>[2x]VSEPTTVAFDVRPGGVVHSFSHNVGPGDKYTCMFTYASQGGTNEQWQMSLGTSEDHQHFTCTIWRPQGKSYLYFTQFKAEVRGAEIEYAMAYSKAAFERESDVPLKTEEFEVTKTAVAHRPGAFKAELSKLVIVAKASRTEL

MYDGF, previously named c19orf10 (chromosome 19 open reading frame 10), is a poorly characterized protein, which was identified as a paracrine-acting protein that is secreted by monocytes and macrophages. Human MYDGF has 142 amino acids and consists of an N-terminal 31-residue-long signal peptide and the MYDGF protein sequence containing a C-terminal KDEL-like ER retention sequence. According to its primary amino acid sequence, MYDGF does not belong to any known cytokine or growth factor family. Treatment with recombinant MYDGF helps to protect and repair the heart after acute MI.

Recombinant full-length MYDGF, lacking the N-terminal signal peptide, was crystallized using sitting-drop vapor diffusion methods. MYDGF crystals diffracted to 1.6 Å. Due to the lack of initial start models, the structure of MYDGF was determined by Hg-SAD phasing by derivatization of a trigonal crystal form using Hg(II)I2. The MYDGF structure consists of 10 antiparallel β-strands forming two β-sheets, which are packed face to face to each other, forming a β-sandwich. The β-strands are connected by loops of 3–18 amino acid lengths and enclose a hydrophobic interior. A single disulfide bond between cysteine residues 32 and 61 of β-strands 3 and 5, respectively, bridges the opposing β-sheets. The asymmetric unit (ASU) contains two molecules of MYDGF forming a close contact. Analysis using PISA suggests that this dimer with a buried surface area of 1726 Å2 may be a physiologically relevant form. However, analysis of MYDGF by analytical size-exclusion chromatography clearly indicates that MYDGF is monomeric in solution. We conclude that MYDGF adopts a previously unknown β-sandwich topology.>UUGCGUCUCGUCGACGAA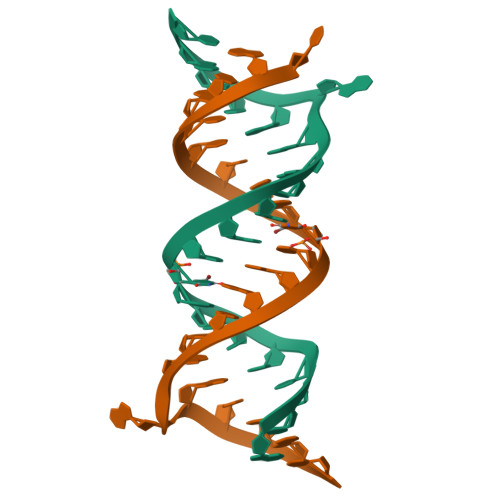GUCGC[4x]> MPKPVANQEDEDPTPYLFVSLEQRRIDQSKPYDSKKSCWIPDEKEGYLLGEIKATKGDIVSVGLQGGEVRDIK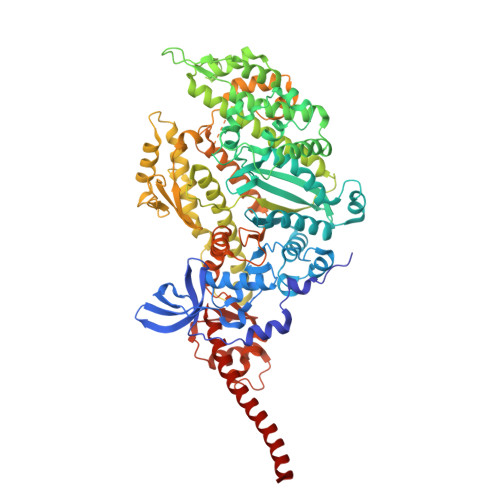SEKVEKVNPPKFEKIEDMADMTVLNTPCVLHNLRQRYYAKLIYTYSGLFCVAINPYKRYPVYTNRCAKMYRGKRRNEVPPHIFAISDGAYVDMLTNHVNQSMLITGESGAGKTENTKKVIAYFATVGASKKTDEAAKSKGSLEDQVVQTNPVLEAFGNAKTVRNDNSSRFGKFIRIHFGPTGKLAGADIETYLLEKARVISQQSLERSYHIFYQIMSGSVPGVKDICLLTDNIYDYHIVSQGKVTVASIDDAEEFSLTDQAFDILGFTKQEKEDVYRITAAVMHMGGMKFKQRGREEQAEQDGEEEGGRVSKLFGCDTAELYKNLLKPRIKVGNEFVTQGRNVQQVTNSIGALCKGVFDRLFKWLVKKCNETLDTQQKRQHFIGVLDIAGFEIFEYNGFEQLCINFTNEKLQQFFNHHMFVLEQEEYKREGIDWAFIDFGMDLLACIDLIEKPMGILSILEEESMFPKATDQTFSEKLTNTHLGKSAPFQKPKPPKPGQQAAHFAIAHYAGCVSYNITGWLEKNKDPLNDTVVDQFKKSQNKLLIEIFADHAGQSGGGEQAKGGRGKKGGGFATVSSAYKEQLNSLMTTLRSTQPHFVRCIIPNEMKQPGVVDAHLVMHQLTCNGVLEGIRICRKGFPNRMMYPDFKMRYQILNPKGIKGIEDPKKCTKVLIESTELNDDQYRLGNTKVFFRAGVLGQMEEFRDERLGKIMSWMQAWARGYLSRKGFKKLQEQRVAL> KVTDALPEPEPPGAMAASEDEEEEEEALEAMQSRLATLR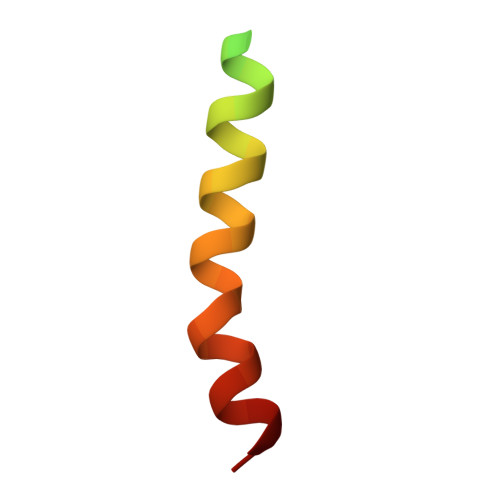S>[2x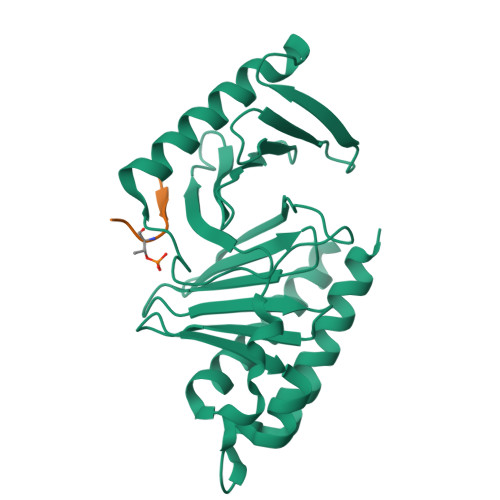]RSMETGEVVDCHLSDMLQQLHSVNASKPSERGLVRQEEAEDPACIPIFWVSKWVDYSDKYGLGYQLCDNSVGVLFNDSTRLILYNDGDSLQYIERDGTESYLTVSSHPNSLMKKITLLKYFRNYMSEHLLKAGANITPREGDELARLPYLRTWFRTRSAIILHLSNGSVQINFFQDHTKLILCPLMAAVTYIDEKRDFRTYRLSLLEEYGCCKELASRLRYARTMVDKLLSSRSASNRLKAS;>KNIFQSTMLTE[2x]> GLWRQSIVRCADNTGVIKACIIGIRNKYGTGKIGARIRVSVRD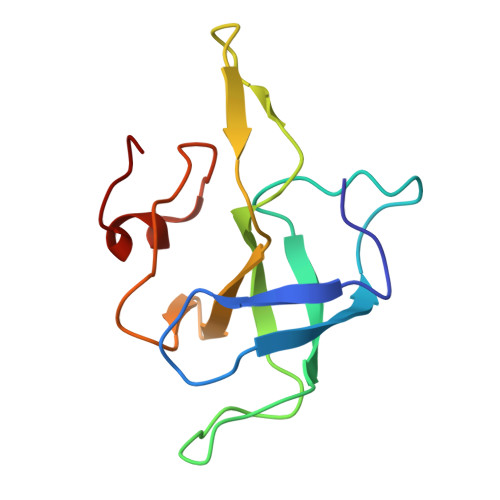KTPECTAPKMPKGVIVRRRKETRRKDGSYIKFDENAFVIIQKNKARGTKIKGPVPMEIRHNCKTLARWIFA>MMVLVTYDVNTETPAGRKRLRHVAKLCVDYGQRVQNSVFECSVTPAEFVDIKHRLTQIIDEKTDSIRFYLLGKNWQRRVETLGRSDSYDPDKGVLLL[2x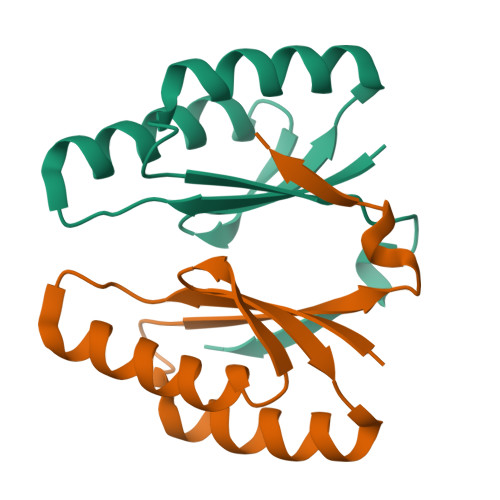]> MNVDLVFLFDGSMSLQPDEFQKILDFMKDVMKKLSNTSYQFAAVQFSTSYKTEFDFSDYVKWKDPDALLKHVKHMLLLTNTFGAINYVATEVFREELGARPDATKVLIIITDGEATDSGNIDAAKDIIRYIIGIGKHSQTKESQETLHKFASKPASEFVKILDTGEKLKDLFTELQKKIY;> EPFWADLQPRVAFVERGGSLWLNCSTNCPRPERGGLETSLRRNGTQRGLRWLARQLVDIREPETQPVCFFRCARRTLQARGLIRTFQRPDRVELMPLPPWQPVGENFTLSCRVPGAGPRASLTLTLLRGAQELIRRSFAGEP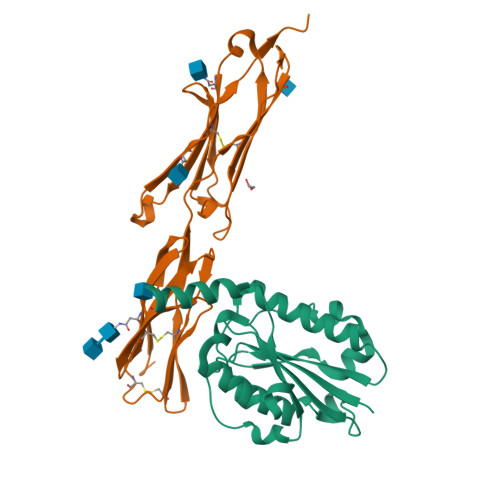PRARGAVLTATVLARREDHGANFSCRAELDLRPHGLGLFENSSAPRELRTFSLS N-((1,4-dimethyl-2-oxo-1,2-dihydroquinolin-6-yl)methyl)benzenesulfonamide | C18 H18 N2 O3 S | 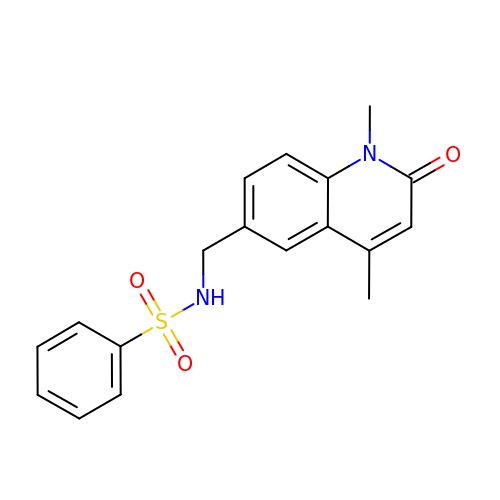JYPYWRMUXLPCGO-UHFFFAOYSA-N>[4x]SMPKDVGILALEVYFPAQYVDQTD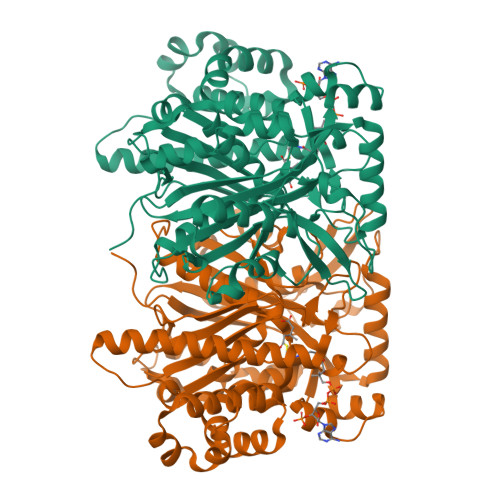LEKYNNVEAGKYTVGLGQTRMGFCSVQEDINSLCLTVVQRLMERIQLPWDSVGRLEVGTETIIDKSKAVKTVLMELFQDSGNTDIEGIDTTNACYGGTASLFNAANWMESSSWDGRYAMVVCGDIAVYPSGNARPTGGAGAVAMLIGPKAPLALERGLRGTHMENVYDFYKPNLASEYPIVDGKLSIQCYLRALDRCYTSYRKKIQNQWKQAGSDRPFTLDDLQYMIFHTPFCKMVQKSLARLMFNDFLSASSDTQTSLYKGLEAFGGLKLEDTYTNKDLDKALLKASQDMFDKKTKASLYLSTHNGNMYTSSLYGCLASLLSHHSAQELAGSRIGAFSYGSGLAASFFSFRVSQDAAPGSPLDKLVSSTSDLPKRLASRKCVSPEEFTEIMNQREQFYHKVNFSPPGDTNSLFPGTWYLERVDEQHRRKYARRPV>PFRTIARLNPAKPKAGEEFRLQVVAQHPNEPGTRRDAEGKLIPAKYINLVEVYFEGEKVAEARPGPSTSANPLYAFKFKAEKAGTFTIKL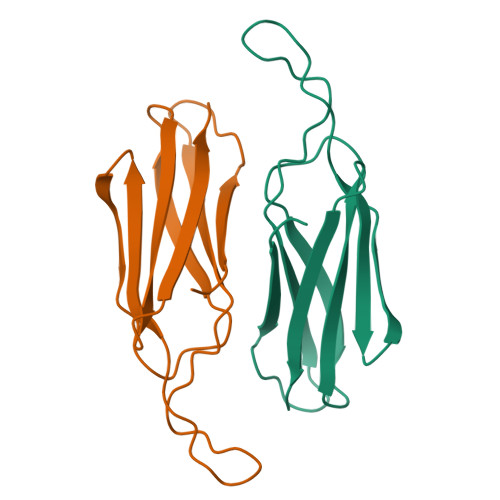KDTDGDTGEASVKLELV[2x]>[2x]MKIQMKTPLVELDGDEMTRVLWPLIKDKLLLPFIDL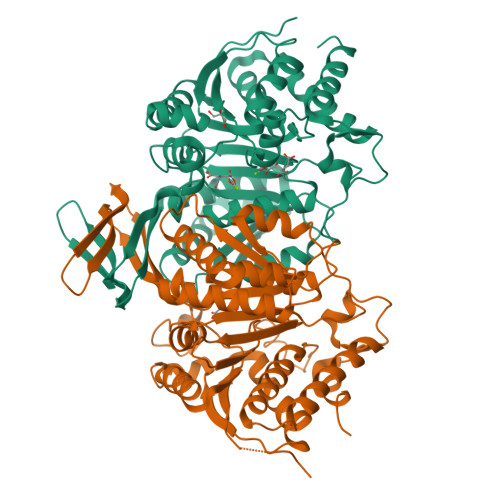QTEYYDLGIEERDRTNDQITIDAAEAIKKYGVGVKNATITPNQDRVEEYGLKEQWKSPNATVRAMLDGTVFRKPIMVKNIKPSVRSWQKPIVVGRHAYGDFYKNAEIFAEAGGKLEIVVTDKNGKETRQTIMEVDEPAIVQGIHNTVASIGHFARACFEYSLDQKIDCWFATKDTISKQYDQRFKIIFEEIFAQEYKEKFAAAGIEYFYTLIDDVVARMMKTEGGMLWACKNYDGDVMSDMVASAFGSLAMMSSVLVSPYGYFEYEAAHGTVQRHYYQHLKGERTSTNPVALIYAWTGALRKRGELDGTPDLCAFCDSLEAITIECIESGYMTGDLARICEPAAIKVLDSIEFIDELGKRLQQLNK> SGMALFSAQSPYINPIIPFTGPIQGGLQEGLQVTLQGTTKSFAQRFVV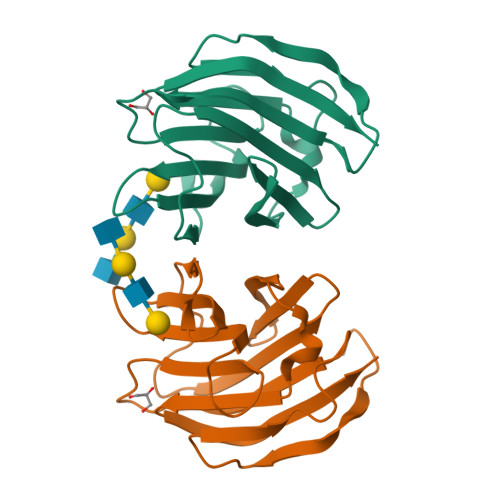NFQNSFNGNDIAFHFNPRFEEGGYVVCNTKQNGQWGPEERKMQMPFQKGMPFELCFLVQRSEFKVMVNKKFFVQYQHRVPYHLVDTIAVSGCLKLSFITFQTQNFRPAHQA>[2x]REVLTGGHSVSAPQENRIYVMDSVFMHLTESRVHVYDYTNGKFLGMVPTAFNGHVQVSNDGKKIYTMTTYHERITRGKRSDVVEVWDADKLTFEKEISLPPKRVQGLNYDGLFRQTTDGKFIVLQNASPATSIGIVDVAKGDYVEDVTAAAGCW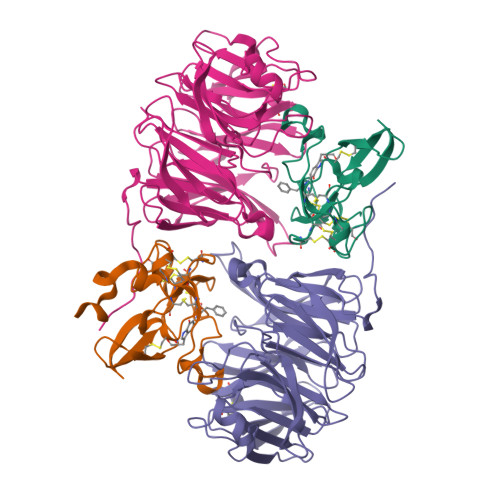SVIPQPNRPRSFMTICGDGGLLTINLGEDGKVASQSRSKQMFSVKDDPIFIAPALDKDKAHFVSYYGNVYSADFSGDEVKVDGPWSLLNDEDKAKNWVPGGYNLVGLHRASGRMYVFMHPDGKEGTHKFPAAEIWVMDTKTKQRVARIPGRDALSMTIDQQRNLMLTLDGGNVNVYDISQPEPKLLRTIEGAAEASLQVQFHPVGGT;>AGGGGSSSGADHISLNPDLANEDEVNSCDYWRHCAVDGFLCSCCGGTTTTCPPGSTPSPISWIGTCHNPHDGKDYLISYHDCCGKTACGRCQCNTQTRERPGYEFFLHNDVNWCMANENSTFHCTTSVLVGLAKN[2x]>[2x]MFKIVYPNAKDFFSFIN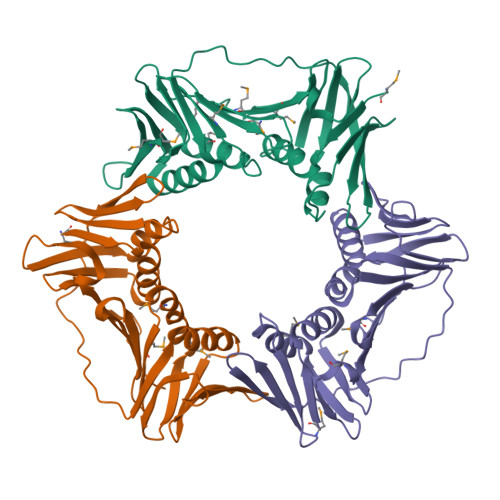SITNVTDSIILNFTEDGIFSRHLTEDKVLMAIMRIPKDVLSEYSIDSPTSVKLDVSSVKKILSKASSKKATIELTETDSGLKIIIRDEKSGAKSTIYIKAEKGQVEQLTEPKVNLAVNFTTDESVLNVIAADVTLVGEEMRISTEEDKIKIEAGEEGKRYVAFLMKDKPLKELSIDTSASSSYSAEMFKDAVKGLRGFSAPTMVSFGENLPMKIDVEAVSGGHMIFWIAPRLLEHHHHHH;>MKAKVIDAVSFSYILRTVGDFLSEANFIVTKEGIRVSGIDPSRVVFLDIFLPSSYFEGFEVSQEKEIIGFKLEDVNDILKRVLKDDTLILSSNESKLTLTFDGEFTRSFELPLIQVESTQPPSVNLEFPFKAQLLTITFADIIDELSDLGEVLNIHSKENKLYFEVIGDLSTAKVELSTDNGTLLEASGADVSSSYGMEYVANTTKMRRASDSMELYFGSQIPLKLRFKLPQEGYGDFYIAPRAD[2x];>[2x]MKVVYDDVRVLKDIIQALARLVDEAVLKFKQDSVELVALDRAHISLISVNLPREMFKEYDVNDEFKFGFNTQYLMKILKVAKRKEAIEIASESPDSVIINIIGSTNREFNVRNLEVSEQEIPEINLQFDISATISSDGFKSAISEVSTVTDNVVVEGHEDRILIKAEGESEVEVEFSKDTGGLQDLEFSKESKNSYSAEYLDDVLSLTKLSDYVKISFGNQKPLQLFFNMEGGGKVTYLLAPKVLEHHHHHH>[2x]GSAMARTEKIYIYGASGHGLVCEDVAKNMGYKECIFLDDFKGMKFESTLPKYD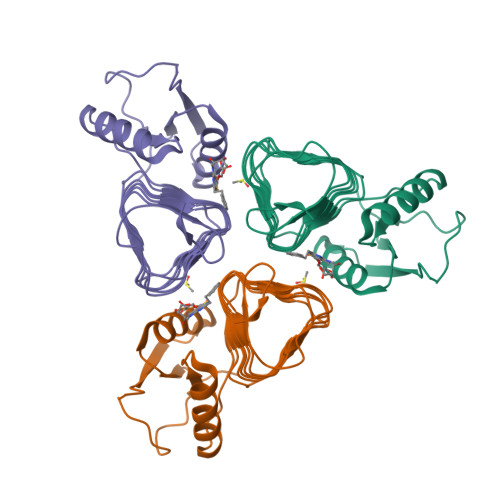FFIAIGNNEIRKKIYQKISENGFKIVNLIHKSALISPSAIVEENAGILIMPYVVINAKAKIEKGVILNTSSVIEHECVIGEFSHVSVGAKCAGNVKIGKNCFLGINSCVLPNLSLADDSILGGGATLVKNQDEKGVFVGVPAKRM> GSSHHHHHHTDPVIAQKAPYPVTVEAGKTYHWCACGRSKAQPFCDGSHKGTGLAPVAYTPDKAGTAY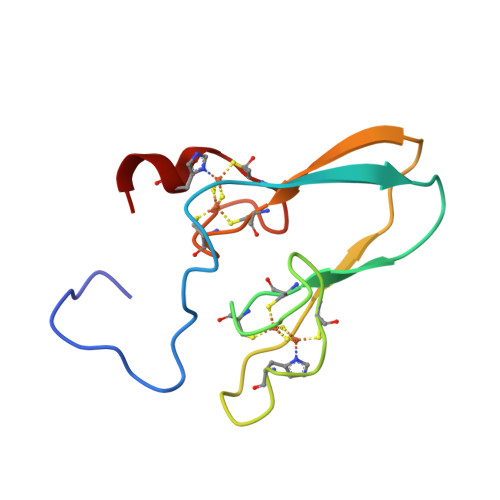FCGCKASKAPPLCDGTHKTL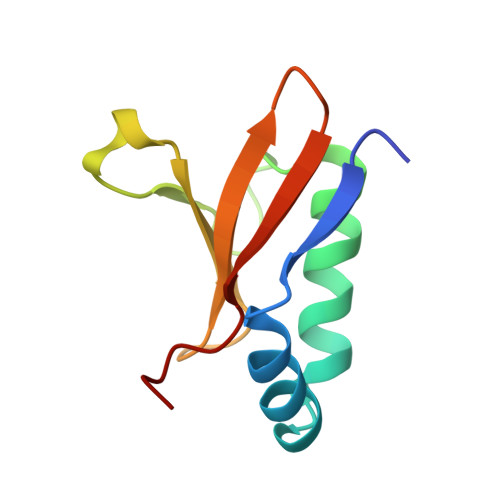> MSNYTVKIKNSAKSDLKKIKHSYLKKSFLEIVETLKNDPYKITQSFEKLEPKYLERYSRRINHQHRVVYTVDDRNKEVLILSAWSHYD>[2x]EPVMTGGPVQGKALWTDYSGMSKEVQGPVSQILFTQSPRTAKGDPYQNYPHYIPEGSRIVLFDLNTKELKVLTNDFATAFDPCTYWDGKKFAFAGVHKKGGGCQIWEMNIDGSGLRQMTDLKGTCRSPIYYAAGSIEEGEGRIIWRDRYFEGDWKEHGMVEKTGMIIFSGSPEGVMDEFHNPYAYNLYRLDTQGGKIIQRITGHVLSGIEFPHLNTTIDQITYNLSSNFDPWLTPDGNILFSSVQANGSRAGGEGRVMICVDNWDGAYPRPIYGNCDGEIGGTSGRSQAKITFGDRKIVYVESPYMNWGVGQLAAVSWDAPFNKTYEKLTGKDGGLYRSPYPLPDDRMLVSYAERGDFGIYWFNFSKCAAGDKVYDDPNWNDHQPAPVYVKYKPRWINTFTAGKNFGVTVVTYQPFDQVKVEGYPHSWGTWICFDTTLSDQPVGPYPHQKAKNVSHGDIKAVRIIQGYQCVEPDSTRFRVGAG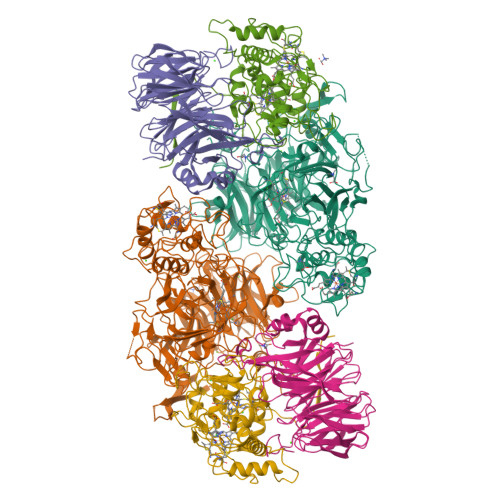AHLLGGERSSSNSGTAFQQRGIIGYQYVESDGSTVTSQLSDVPYYMQILDDKGMSVQTALTWAYLRPYHGRICSGCHYGSYRGRAFKNIHAKALYNWWYDDRSHYDSPFAFRYLKFDNDGNYKGVKHGEDVVVPSDIYYGGPSGTTSQPVEGLTLDKQRTVDFRRDIQPILDAKCAMCHDSNNPPNLGGGLELVSVDGIAAYSRAYNSLLEPQRGKDPNIGGKYVNPSAAINSLLVWRLYEAELSANAPREKIFPIEGRLLHNKFLTQDERYAIVEWIDLGAQWDNIPGPDFYPGYLVK;>GYIQGTHVKTDLPGPFHITMSPDGSTLFISNQSGHSVTFVDARTQKVTGEVAVRVQPEASAVTPDGAFLYVCNAESDSVSVVDIQRKQEIKEIKVGDWPSGIKISPDGKTAYVACSGCMWNAIDVIDTGRMEKVRSIYTSDYGPRMVEISPDGKTLVAILDTVGSINRSVDFIDIASGRVVENRVIHESSNLRDVVYTPDGKYIAVTHQTPKNWLPVCEAENGQVFTNNVTIIETKAGGKVARLPLDDLNNYDGNPYGMAMDPKGKYLYIGVRGMHRVTILDMDKVLGLVRSSTQEELDYLRDDLGLVRDYLVARVPTGLGPSSVCLSPDGKFCYAANYFSNNVTVIRTAVD[2x];>[2x]GQPRVISTIQTGATWEPLGREEPLTVPEVHFRVKHSPFKSELVRYGQFQFNDAAWSLQGSYSCASCHYERGQTTGLIWDLGDEGWGSWKNTKYIRGGRYLPPFRHEGFTGHPDEIVGATSSLDRVCGRDPGFVFRSENFSPMRLEALICYIRALEFTGSPFRNADGSLTEAQKRGQKIFEDPKVGCLECHPGDPMDPRALFSDAQTHDVGTGRVGVNGFRSTPGKVFNISALEAGEDPYGVESNTPIIGLDLVKEFDTPTLRDIYASGTYFHDGGARTLMDTINNTVNDKDMHGRTSHLKQQELQDLVEYLKAL N-[2-({6-[(2-sulfanylethyl)amino]pyrimidin-4-yl}amino)ethyl]propanamide | 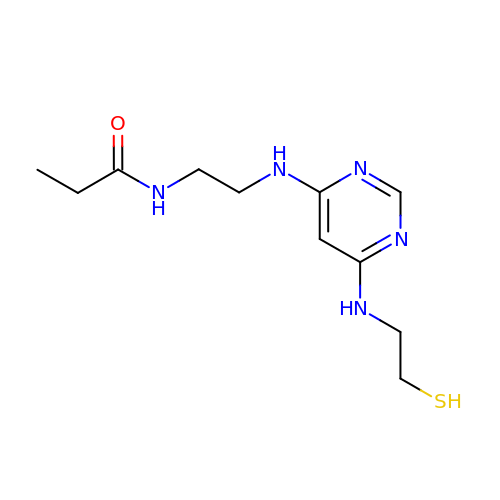C11 H19 N5 O S | MXLYIGOSAJROJY-UHFFFAOYSA-N>[2x]SQNGVQMLSPSEIPQRDWFPSDFTFGAATSAYQIEGAWNEDGKGESNWDHFCHNHPERILDGSNSDI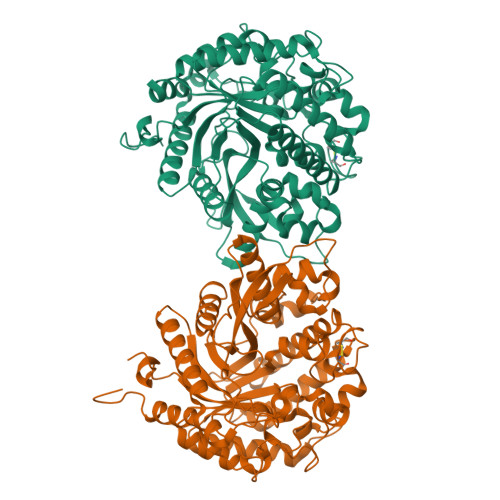GANSYHMYKTDVRLLKEMGMDAYRFSISWPRILPKGTKEGGINPDGIKYYRNLINLLLENGIEPYVTIFHWDVPQALEEKYGGFLDKSHKSIVEDYTYFAKVCFDNFGDKVKNWLTFNEPQTFTSFSYGTGVFAPGRCSPGLDCAYPTGNSLVEPYTAGHNILLAHAEAVDLYNKHYKRDDTRIGLAFDVMGRVPYGTSFLDKQAEERSWDINLGWFLEPVVRGDYPFSMRSLARERLPFFKDEQKEKLAGSYNMLGLNYYTSRFSKNIDISPNYSPVLNTDDAYASQEVNGPDGKPIGPPMGNPWIYMYPEGLKDLLMIMKNKYGNPPIYITENGIGDVDTKETPLPMEAALNDYKRLDYIQRHIATLKESIDLGSNVQGYFAWSLLDNFEWFAGFTERYGIVYVDRNNNCTRYMKESAKWLKEFNTAKKPSKKILTPA> MGSSHHHHHHSSGPQQGLRDIVPDETATEKDAFANPRAALRYLYSCYGYLPQSNMVQSCMDFTGDETISPFAESYVKFAEGSYDSSNTIISYWNTLFQGIRQCYLLKENIHSVPKISQEEVDLYTAEADFLIAYFHLLLIKCYGPTI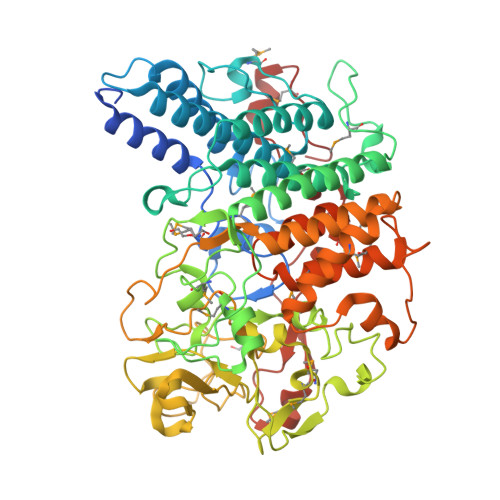LVKELPALDTPAENMLGRRPYDECIDWVADLLDDAATRLPATRNSSDYGRATSVIAKSLKARMLLYAASPLFNGNPDYTDFKNPDGEQLMSTTYSEEKYKRAADATWDAIQAASGAGHELYIASTTSNAYPEPTNLTERTLRMTFMDSENYKEVIFPETRKAGAYGIQRKSIPFFPRGSWNGIAPTITMLDRFYTVNGLPIDEDPEFNTNNKLDIVTIPEGTTYAEPGKRTLYMNMNREPRFYAWVAFENGYYECRTDDKRYAYHKFWGAERSEGDKWLTGFLATENCGVRADDGKIVTAARSQNYSKTGYLNKKGVHPGIQATVGTPGPTVEYPWPVIRLAELYLNYAEACVGYGKEGYPEKGMAYLDKVRERAGLKPVLESWANAKVPLTSYDGQCGPDGRVMKIVRQERMIELYQENHNFWDIRRWKMGETYFNVKARGLNILAETMEDFAKIVEIQDKRTFDAPRQYLMPIPAGEVSKNPNMVQNPGY>[4x]GDITHMASMTGGQQMGRDPMRICSFNVRSFGESKQEDKNAMDVIVKVIKRCDIILVMEIKDSNNRICPILMEKLNRNSRRGITYNYVISSRLGRNTYKEQYAFLYKEKLVSVKRSYHYHDYQDGDADVFSREPFVVWFQSPHTAVKDFVIIPLHTTPETSVKEIDELVEVYTDVKHRWKAENFIFMGDFNAGCSYVPKKAWKNIRL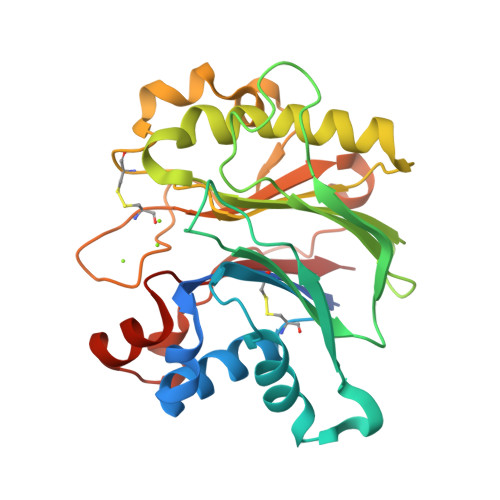RTDPRFVWLIGDQEDTTVKKSTNCAYDRIVLRGQEIVSSVVPKSNSVFDFQKAYKLTEEEALDVSDHFPVEFKLQ> MAVVYYLLLAGLIACSHALAAGTPALGDDRGRPWPASLAALALDGKLRTDSNATAAASTDFGNITSALPAAVLYPSSTGDLVALLSAANSTPGWPYTIAFRGRGHSLMGQAFAPGGVVVNMASLGDAAAPPRINVSADGRYVDAGGEQVWIDVLRASLARGVAPRSWTDYLYLTVGGTLSNAGISGQAFRHGPQISNVLEMDVITGHGEMVTCSKQLNADLFDAVLGGLGQFGVITRARIAVEPAPARARWVRFVYTDFAAFSADQERLTAPRPGGGGASFGPMSYVEGSVFVNQSLATDLANTGFFTDADVARIVALAGERNATTVYSIEATLNYDNATAAAAAVDQELASVLGTLSYVEGFAFQRDVAYAAFLDRVHGEEVALNKLGLWRVPHPWLNMFVPRSRIADFDRGVFKGILQGTDIVGPLIVYPLNKSMWDDGMSAATPSEDVFYAVSLLFSSVAPNDLARLQEQNRRILRFCDLAGIQY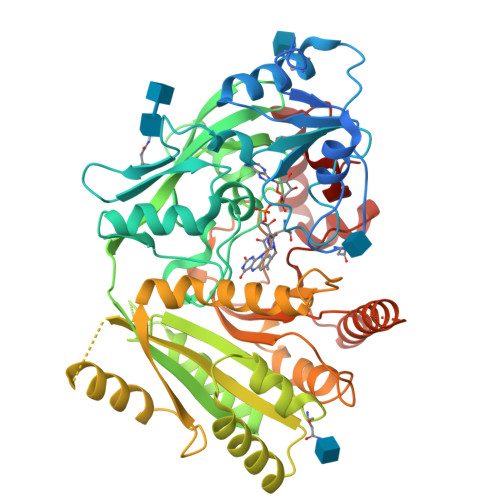KTYLARHTDRSDWVRHFGAAKWNRFVEMKNKYDPKRLLSPGQDIFN> MEVKELERDKNRVVLEYVFGAEEIAQAEDKAVRYLNQRVEIPGFRKGR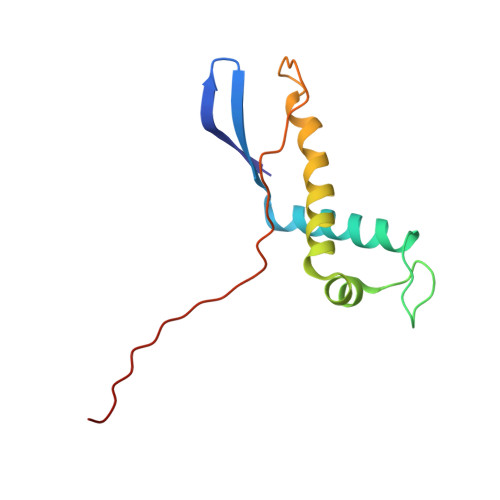IPKNVLKMKLGEEFQEYTLDFLMDLIPDTLKDRKLILSPIVTERELKDVTARVVVEVHEEP>MPKIYTKTGDKGFSSTFTGERRPKDDQVFEAVGTTDELSSAIGFALELVTEKGHTFAEELQKIQCTLQDVGSALATPCSSAREAHLKYTTFKAGPILELEQWIDKYTSQLPP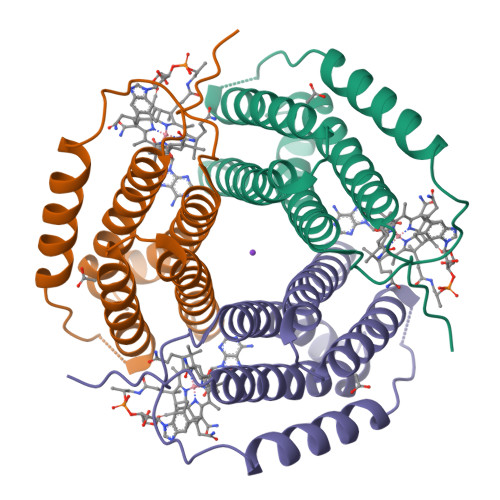LTAFILPSGGKISSALHFCRAVCCRAERRVVPLVQMGETDANVAKFLNRLSDYLFTLARYAAMKEGNQEKIYMKNDPSAESEGL[4x]> MNPSQTQKGKIQIQVSRGSIDLLVRTMYEDINNIKLKNERFQKKKRAEDERRRRERYAEIQQEAIASGKKNAALEMKWAELKELDECEELNREMQDQQQTFQQIIEGKENLRKEFEEELKRKDDEYVKMLKEQSNDIKDMISKMRSQFYKIRDANMQELEDIERHFEQERSNLLNEFKAKIQATFKKHLDLEEQYVKEHAKTEEEQTKNIEDLRIKGAKHYAELKITMETEIQDLEKCFEDMKALYQLITEKLDYSLKVLQEKFHENNSMCDELKRKENNFKNRLKQLTKDYKQYDKKFKLENKNLTQEYKRIIRQFKELQKKFKHFEKADLDKYSEIQKMNEAEVKELKDKIIKCNITIHIQQLGMQWIPPQSEEEILAQQKLQLEQGGKAEEEEEREFEFCISEIKIGEICNIILEEADFLIDDKLREELEGSAEPEQIFQRLDCIKKCLYIDSEDEMNLFFRELITKCRVKSAEEIEEEARKQLLLLGLIKEAEENENPEGEEVQQQEGAQQKKKEEGNKKDDPKGKEGAKDSKENANPQGQNKSNQDERKKKKDGQDDHAGQGQGQYDSNQGGMGENQEEGENAEGQENLEGEIEKEIDLENTQINLNEVVKFLQNWQANKDKRKEKLEKESSKKAVKQETEREKKERIAREGKKYWEKLTQVLPERTFRIWNVNFFKFSFEKQILLNQINKLRFWTDLCPNIMNFFWTDKNQSKKPVNCITKMKNQRIFQINTYKLIMNLLSALQDSLIQIKDKDDFIQTKISTNLFTFHNFQILLQIFIVNQSFLFIRLCQSYSKKIILLIKNINQKLFNLSNFKNQFSF;> MALLGKTLKGRSTRPGGIPQKRNIKWRQLAKNQEEFDQLKQLAKMKREGLKARIKDEQKVVTFNKKKLITYWRKIMRIAKTEQLKNEIDIYSQNNQRELDSKEAFIQMLDKNLDEAEDQFQIALRNHLIHIENLMQLQEARMRGLAEEFNRDVNILETEFDLEREEMVKTHKTQLKELEDMIETVKEEDKKKTEEAQNEFSQFKEETKNKNLEETNVMKIILETKQTKYYTELEQMNSKFQSDTSNKVKDHQFYHAHNKNRKQEIDRYLRTISSKKAKIDLMKLKILQHCKEFNARNSALKKEKENISRNYHELKLKMQKFREEESRRLKELSNNSRNAVLKLREYCALGEKILKTAELCRRLETEKEKVLPFYESSVDEDQIPEQLKNEFEHLKKEDAEEYAYLNNFYKRYNKVLLDKLAIEKQKENLQRDNQLLKSLLKQYLDGISLNDDVLKNENNPLLVVNHKFNLGKMPVEKIENKTVIEGVFEVRNTSHQLQGQRAPPFQ;> MSKAAKAKKNVPVVSKLEADARKAAEGVNDNESEEFKKAMRKEARALVEQFNEEKKLLAFYQQERQKINYNWIIAKKELEDKKSELINKEREIQDLQENHFMTLNVYKQKIKHLLFQNQDQQSELKKDVEVTLKQLEDQHRIKSRELKTDVRSLKVTKKEQEISQQDYLFALKSEHDKQMTLMRQDYERQVNDIKRKYDLKMQNLTKEMEEARAAMIKQLEDNKNQKIAEIIKEHTQKYNDIKNYYSEITATNLDYRKTLKNEIKELQTKDEEYKKTLQQTEKGYKELNEPLQALGIEIIQLKKQDEEQEAIIKEKEELKQKIDNQERLFRKLEYEYEVKLQQFQYLERERNALYAKFNQTVFEIHQKSGLENLILEKKVTNLREDLEIKDLQIHQVLTAANIDPNSVGSINKSLEEVESLKNELISELQAQLKQIRKAHSHMVKAYEGKLSEFVIPVEELGFDPLVPTNTD;> MPPKKAKGKKKKEEEPDDEYKSMTGADLTQTLEKLKERVNEMRTNRNYIQMDRDMVENFYHNTLKEISEVKTKISNKETEAEEKESKHRIDVKVFLQKVKHLEYEQEKSNLNIEDDGKKAKEKEDAYFEDITKNMKQLKTQLKSEYLEKEKANIQQVQEEKKDHQSLLKIQQKKFDELINNLIIKYEERLAKLKEDLELKLKVEIHELEERKNLHINELMNNHEKAFAELKKYYNDITAENLNLIKAHKEKIAQIYANIQLNTKNVADNQAKNEQLKEPLAKHREIRNKLKEDLKQFAKHKMSLQNLKSKAITLKDKITKLERDGKDLDEKYEKVVREKQELEKKFEDITQEVKKNADLNNNVLSNRLQILLKEYNNKEEELRTIIDNAGLDHNLHEQLKQRVQQSIEAKNTLIKNLKYSIHHATKAYNDAIRVYEAKLVEFGIPIEELGFQPLETITSSMPAGLVSS;> MATTTNILHDVVRDQSMVNYVSNRDRPLYFKRPLVPQMTDIPLHISRPPVDQQVDYQTMQMQQNATIVEAPTKDAFVQTDYRESETQTDPYTPKCFVRDGDHPEVMELKDYKYGKGLPASIEELEQIELNREKVWFENSLPPISDEASFNLRRKLMEEQELREWSKKENEIKKFQNEKLYLLQQALIEREKEVEDKSQERIEEIRQQKTEHKNRQIAKIQRKKIKIDRKMTKSRKMQGKETLKRDIIEDYANFASRVYAGITHEGLSLDKIANKYEVQPLALGNYEMLQALHEGIRPREFETRVNLKKEIKEIEKNYTRLENYHRGELKKAQDEINGVHEQSKAQQKQEGNNFSYRNFENKIRPATPTWKYDTDFNISPSLITEIQEYRGPNGVQLMQAADKREEAVLLLQRLLRGRTTQNIMYEGKKKRTALIEELLTVAQIENLEEDKAEEVLMQQHEEKVKNAVLESIQGEVIAETMDELSKELLRIKQERKIQQMVEIAEKDRRIREIEEAGKRQAEEILRDREDVLHNQLIRVHQGTVDTYLDWLMSNALEQSSARQATIMTNLRKAKFNLPLEDFERKYNNNQTLIKDLVHSFLIPNVQRSKLKKQIQLEEKRFSEAAKRSLQQTITRASNKHANVQN;> MDQGEFIQDDNDQDYDQQEGDDENNDYMEDPQQDNNYNQNGDNLDDQGQDDDGGQNNLQQPSVPPEDDEDDDDDFPEYANEQNKRLNEIIKKKRKLIKDISAKIEEKSDRTKVLQEHLKNVEQELLHTQALIDAKNKEIETEDHMKQIAERQSGRIQSELKILEKRSIEQQEKLNDVQNQIFRGNEKMDQYKLEMNWNQEELEQWALAARQKEEDNLTLEKYKRADEVKIKELNLAIEKLTAEVGRKQNELEKEITETQAAQIELDKTAEEFKRQHEERHKLFLQWQEVTEIISKRDLAIREEGENFARIKIEIKSNKDALEERKRILKEAKEENKRIQMANELMERQNIQQISDNKHIEEQLAEKKADVEILKNQVSAFASDLSSKKNRIAILSQELLAKKQRLNAAQKKYQAHQVKLKNEEIMAKQYENDRSYAEEKYRKNEKEKKELEKEIRTQKENLFKHTQELFKHREREANLYGEIQGNMAACRNLQSHITKLNQEFQRQQELLYNAEYQIQLMERRVARAKGERTLEEKKDLENEIMNAERELGGVTGQNKELIESLKNLDDEIRTVKKKLAYVEEENTKYSSLIEELILENDMTYQDLNKIIKQKEEVLVQHDTMKLEIKKINESLNGATEKVFNLENQIYQLEMSMQEREKEIEVHKDVLMTEHKAAEEERHKIAVELAERKNKVKNLKIKYESLVQKNKASNGEVESVHEHSQAYYVIKAAQEREELQRKGDELNAKILKNEKELKALDNTLNHLKNRNSNYRDKFLNKGVTTQHREEAEGLEEQCRAASQNLFKKRDELQKLQKEQEEDTRRYTEIKNKLERLYEQHQSLDQEISKYQKDIDQQGDKLQRAQNSLQRNYQLAVNKNQNFINPKNPH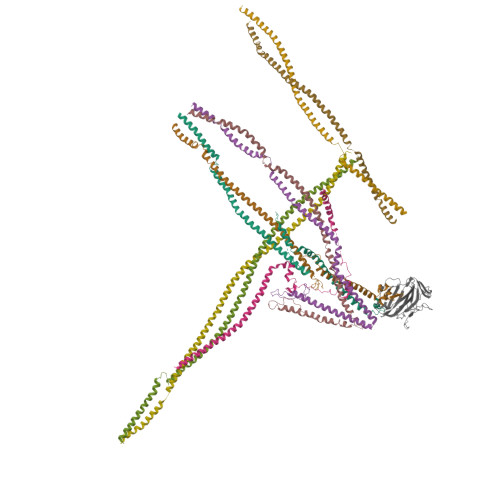MIQVKLDNQNNLYKTLLQGLYSLQQDIPELSSVVDEILKEQRIQNNKAPSSIDINSKRSSQSGRSQRSQRSNISNQ;> MSNQQGPEDNNLEDDMAYLPADHPLLAKLQIDLTKQLTDEHERVDQKLIEIDANLKKLEKTKEDIGVRLYSVQQQLAENQMNFEQAHENYNWVQKLRIEAEQKLKTESEVYDAKKKELEELRKKYLKAQDELSKLTRTLYQINEFNQQMKGQIINTKTNTYRAEENVVNLEAQKKKQDLLIDTMNEEIKRQTEQKTILTAQLISQKEETEQAKQILKEAHLEMQKIIASKKNLLERWQKSLMTMQRMDNALQAIKEALKGQQELNLQIGTELNGVNAEIRKETEIQESLEGKNKKFDYEKDYLQKKYNELQEEKSKLEAQINLLTQSLRQTETEAGRAEIDKRNIEDQMNLIETNIMKLHTETKKLWEDLVHQKSEHTTIEKTATNLNKQANQISIEIEDKSVELENLLNEIARVKIDQLNTLSQIEVLENKRREVIKEREEKEITVATYEVQIRQGHDLNEKKQHEVGRLNREHDKLSSVQSDMSRGPLEAKRNNLIRKTQELGKENDLMQREWIKKQTLLVTQNNRLNKIEEDVSQLKTKQTILEQKKLRLNNNYRIYEKDIREIQNALKNLRNEMNKLNDAIYRNKEKQQKLDNENFNIKSEFVEKLKELEKESVKLEVEIDRLKEEKADLLAEIVESERQILLWERKIQLEKEMQDALDPTVGQTEIQELKREIHRMELRLDDLRKKQEAIIAEMERAVYKRETIQLKYMNKDKTFSNSNSMSQKSSSISAASDNSAQITKKIAQLKTTLNQTTRNAEQMEKAIKNKKIELDDLNAQIEGNNDNLQKLESDCYNKNIELTKHKLERSTNILSISCMQNKAKKLEDLVAGKARLSVPEATLMTKYEELRDKNQEIKEALQKLCDDAPQYVEVLNYLIDLNVGDDDEDQEQ;> MASEDGEMPSQFEGIDPEQLTESQMQQYMMEMQRQGLLDSNMEGGQYEEGYEEGQEGEGYGEEYGDQDYDGNQNEYDSQQDSQQQGHDQVNEMHQDRYDRRVNSEISGNYEADDETLRKIRRDLLDNINLERRHRDLQPVYIDLTTNNISQYYSEYLVNNEHNQDFYENAKVRYNNLGECELCHITAKFEPDADITKEYIYDYFMEIGYLFLESEEEKRIILNPANNHIGIGVFFDEIQIVVVLILSEKVLCIQKISQPEQNKIEIRGKMLDENFGIYAIRIMNVDDQKKDIKGVGPEFIEYTRSTQEWMASFELELYNQDRMAIEYYTRVSPDSIPYKKKQSKNEKLTYKHLQLRLRTPFQIYPDPKYAAEDEKERIRKEQEILAHEEQERKEREENDAKRLKQSRKDYGDGQYDDDEHGQDDFNSQSDISDKDKHHDSMHAEQEQNQQAAQQQQDTISNKEIRQELEMAITEAQRQHDEFMLQNHKLQEEIKLLKNKNDGFVDRSNETAMNEHKYLNTLAHVHQIRLDLKQTQTRYNQMSQELQKKLEQKQKKCNEIKYAFLELKREVAKKAANSRTDKPIPEQQINEWEKAELQKSKELQELRLQILRLRNAYVKNQKILKKKEELAEGLHLIDFEQLKIENQTLNEKIEERNEELHKLKKKNTTTIQILTHTREKLGFVQGENGELNSQNVRKDQELDDMRKQLTQQKKTKDKLRSVNLTLKQQTGIVNSEELGQDYRDLRTRVSKLEEEKKRLEQKLRSMHEAIKTANQISTQNMQSQNNSLKKPYQPY;> MNQDKHPEITDEEQELITVEELSQKLELLYKDMEQIRRENLLFEAYLARNRKEIAKEDEVSEDKKGKGKKKDKNVDKKSLLLTNEEKFEIAQQEQDALKKQIDDGRIKSDQILETLRAILEETDMAITEIRKDAFDFQREILVGGENSRTGKIEAEKIIKFFEEKERQKDALIAKYSSKRTNLERQILKTNNQIQKKEEMGDDLKFIDFYQLQIENKKYVKEIDDKNKKLLALKISTNRISQTLKDEKQNLKQELDKGKEYASQMSERKKKISKIDAQIKSVKKVTSKLEKDRKIYDKQKEIFVQDNQDDVPQIMKYVQYKSKEQQLLYAIQNLERKIEIAELAYKKANRILQSSQQFQQK;> MFKNTFQSGFLSILYSIGSKPLQIWDKSIRNGHIKRITDQDILSSVLEIMGTNVSTNYITAPADPKETLGIKLPFLVMIIKNLKKYYTFEVQVLDDKNVRRRFRASNYQSTTRVKPFICTMPMRLDEGWNQIQFNLSDFTRRAYATNYIETLRVQIHANCRIRRIYFSDRLYSEEELPPEFKLFLPIQGQNKTNV>SSPSPLNPGTNVARLAEQAPIHWVSVAQIENSLAGRPPMAVGFDIDDTVLFSSPGFWRGKKTFSPESEDYLKNPVFWEKMNNGWDEFSIPKEVARQLIDMHVRRGDAIFFVTGRSPTKTETVSKTLADNFH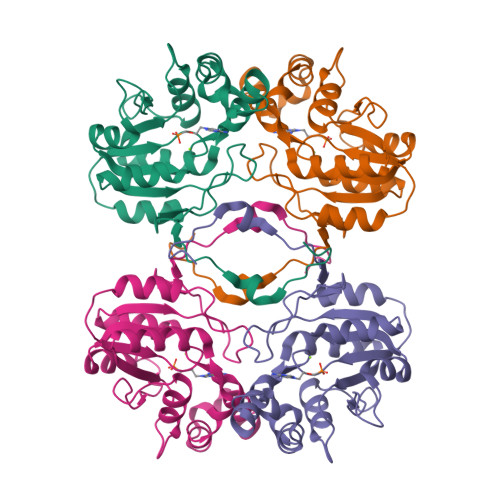IPATNMNPVIFAGDKPGQNTKSQWLQDKNIRIFYGDSDNDITAARDVGARGIRILRASNSTYKPLPQAGAFGEEVIVNSEY[2x]(3R)-1-(3,4-dihydroxy-9,10-dioxo-9,10-dihydroanthracene-2-sulfonyl)piperidine-3-carboxylic 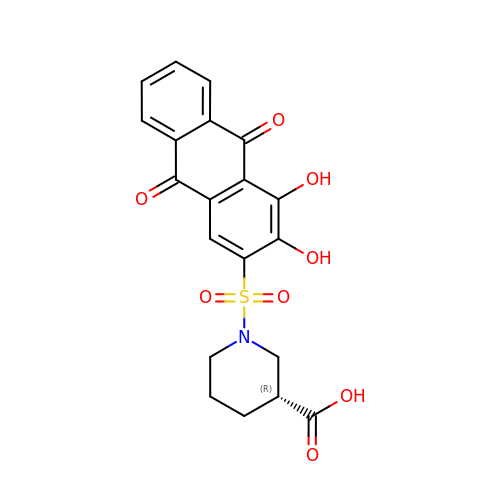acid | C20 H17 N O8 S | COKUEECTCYPUSI-SNVBAGLBSA-N> T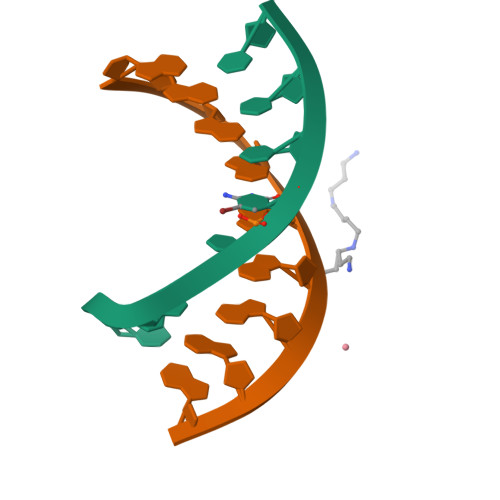TCNCTTC;> GAAGAAGAA> GASSRLRSPSVLEVREKG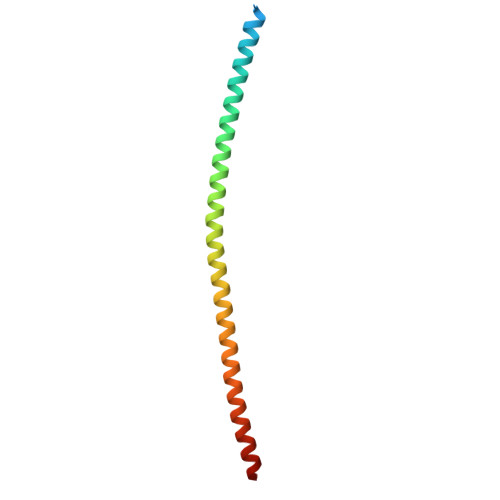YERLKEELAKAQRELKLKDEECERLSKVRDQLGQELEELTASLFEEAHKMVREANIKQATAEKQLKEAQGKIDVLQAEVAALKTLVLS> HHHHHHAGQPEPVATPPAVDCATTKCVALTFDDGPGEYTNRLLDELSEQHTPATFFVLGKNVKKYPKTLKRMVDEGHQIGSHTFDHKDITKLTAEGIEHEVQWTDEAIEQAAGVKPQILRPPYGAHGAVYDRLIPYPLVLWDVDTLDWKHHDPQKTVRIALEEAKPGSIILMHDIHESSVKAVPQLVSKLHDAGYTLVTVDQLFAGTDFKPAKAYDHRFKTNP

CE4 enzymes are capable of removing acetyl groups in chitin, chitosan, and CHOS, thus converting GlcNAc (or A) units to GlcN (or D) units. The protein has a somewhat deformed (β/α)8 barrel topology that is characteristic for CE4 proteins. Next to CHOS, ArCE4A deacetylates chitosan, chitin and acetyl xylan. X-ray crystallography yielded two structures, one for the substrate free protein and one for a complex with (GlcNAc)2 bound in the active site.

The structure of ArCE4A without (GlcNAc)2 comprises residues 42–241, meaning that no structural information was obtained for ten N-terminal residues (32–41) and five C-terminal residues (242–246). Note that both the N- and the C-terminus are located on the opposite side of the protein, relative to the catalytic center. The structure contains a Ni2+ ion coordinated by Asp56, His105 and His109, which comprise the metal binding triad that is conserved in CE4 proteins. The Ni2+ most likely originates from the protein purification by nickel affinity chromatography. The Ni2+ ion is in an octahedral arrangement, involving three water ligands and the metal binding Asp-His-His triad. It has been proposed that one of these water molecules, coordinated by Asp55, is the catalytic water acting as a nucleophile during catalysis. Superposition of the two ArCE4A structures reveals that the water molecule coordinated by Asp55 in the substrate-free structure indeed has a position that could allow it acting as a nucleophile during catalysis. The other two water molecules, which coordinate the metal ion in the substrate-free enzyme, occupy the same position as the oxygens of the acetyl group and the hydroxyl on carbon 3 in of the sugar bound in subsite 0. It is worth noting that the superposition shows little difference in the conformation of the above-mentioned amino acids.>GTMGVNAVHWFRKGLRLHDNPALKECIQGADTIRCVYILDPWFAGSSNVGINRWRFLLQCLEDLDANLRKLNSRLFVIRGQPADVFPRLFKEWNITKLSIEYDSEPFGKERDAAIKKLATEAGVEVIVRISHTLYDLDKIIELNGGQPPLTYKRFQTLVSKMEPLEMPADTITSDVIGKCMTPLSDDHDEKYGVPSLEELGFDTDGLSSAVWPGGETEALTRLERHLERKAWVANFERPRMNANSLLASPTGLSPYLRFGCLSCRLFYFKLTDLYKKVKKNSSPPLSLYGQLLWREFFYTAATNNPRFDKMEGNPICVQIPWDKNPEALAKWAEGRTGFPWIDAIMTQLRQEGWIHHLARHAVACFLTR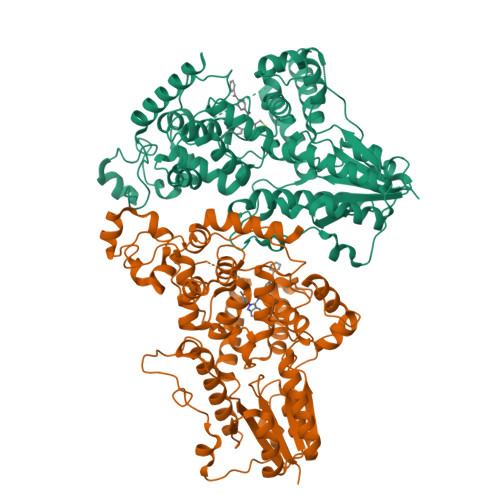GDLWISWEEGMKVFEELLLDADWSINAGSWMWLSCSSFFQQFFHCYCPVGFGRRTDPNGDYIRRYLPVLRGFPAKYIYDPWNAPEGIQKVAKCLIGVNYPKPMVNHAEASRLNIERMKQIYQQLSRYRG[2x]> SSDLVAPSPDAF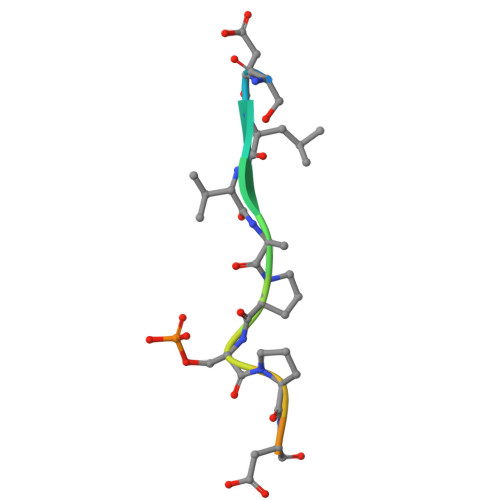RST> M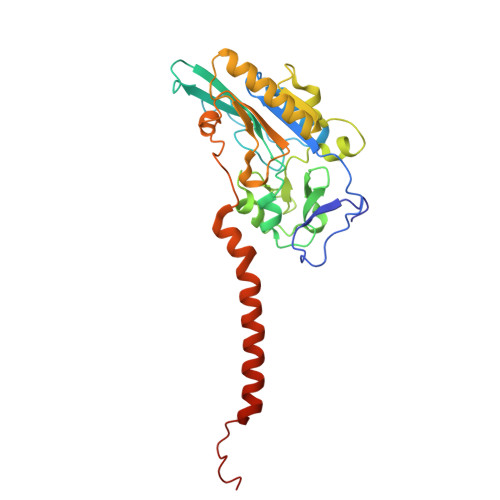AMETQDIIKRSATNSITPPSQVRDYKAEVAKLIDVSTCIGCKACQVACSEWNDIRDEVGHCVGVYDNPADLSAKSWTVMRFSETEQNGKLEWLIRKDGCMHCEDPGCLKACPSAGAIIQYANGIVDFQSENCIGCGYCIAGCPFNIPRLNKEDNRVYKCTLCVDRVSVGQEPACVKTCPTGAIHFGTKKEMLELAEQRVAKLKARGYEHAGVYNPEGVGGTHVMYVLHHADQPELYHGLPKDPKIDTSVSLWKGALKPLAAAGFIATFAGLIFHYIGIGPNKEVDDDEEDHHE>MATKTSIHPSVNELYQRLAEDQLSNCFDRFDPQEKIRCNYCELGVSCQLCSNGPCRINEKVGATLGVCGINADGMAMRYMLLRNVMGTSTYTYHAYEAYKTLKMTALGNTPFTITDKDKLYQMAKDLELNTEGKPEDVAVRLSDFLIWELYRDYDEPGKMIEVYAPLKRKEVWRKLGIYPAGPLHELKDAAASCLTNVDGDYVSLATKGLRLGLSCIYGAQIGLELVQDILFGTGMPHEMDVDLGIFDADYINIVFNGHEPFVGVALILAAKEAVNQDKAKAAGAKSLRIYGSIESGQEVVQRFQKDEVFRGLTGNWLTIEPMLATGAVDVLAMDMNCSPPNLGPLAEKYGATLVS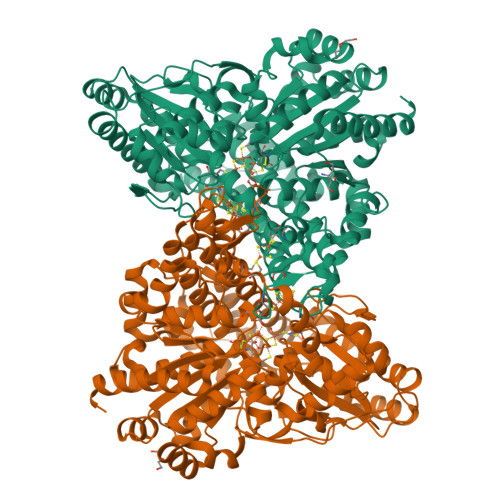VSRLVRFPGIHHFLDYKPSEVREIAQKIIDIAVDSFKNKRHGKITPKIPANIQKAITGFTPEAILKALGGSINPLIEVIKAGKIKGAVGLINCTTLKNGPQDYVTVNLAKELIKRDILILSGGCGNHALEVAGLCNLDAINLAGPGLSEVCRNLNIPPVLSFGTCTDTGRISLVVTALANALNVDTADLPVAVTAPMYMEQKATIDALFALAYGLYTHVAPDPPVMGAPNLVKLLTRDLPSITGGRIAVGSDPVKVADDILAHINDRRAKLGI[2x]>[2x]MKPHNSEKYFVKNGQPHFLISGEVHYFRINPKLWRNHLQLLKQTGADTVSTYIPWDWHEIEEDDFDFEGKTHPARNLIRFIKLCKEENLDLIVKPGPYILAEYENQGLPSWLLKKLSKNAFALDENGNVISPDLVSYLSDEFLEYTFKWYDKVMPIISKHQKEHYGPITMMQLCNEIGVFQWLSGKSDYNPKVINLYKEFIIQRYKTIEKLNSVYSTNYNSFDDLKAPSGKIKLRSDYCAYFDFHLFFREYYNKYISILKNKIRSFGINIKLTHNIPGWIYGNASELPMLISTYSEIMKNHPDIIFGLDHIPEFVSFRNAHSDLACNKILEAMQPEAPVWAAGFQAGTREHHVKAYAKDLETFYIASLAHGIKGF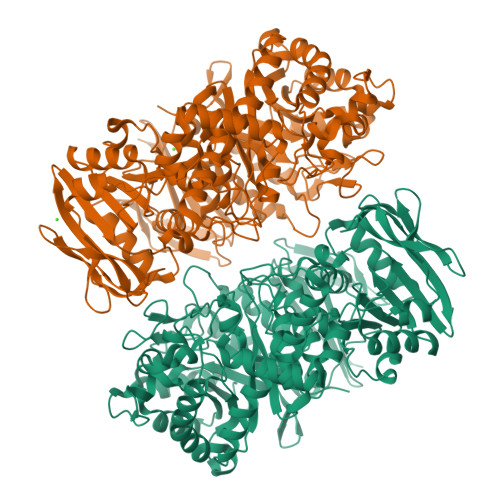NYYMFSQGINPEGKGFYGKTFYFQTALDAASNKLALYDSIKKVNRFIRKEQKDLLRTNVNSEICVGFYKPYFFTELISSQLLKEKKLNVEELGLYIDPRFLREEILFNGLLRGLQTLNYNYDVVDLENCDLKSLTAYKQLWITSAEFMDAETQNLLSEFVLNGGNLILYPAVPTLDNYLNRCEILKNNFGIEFITKDSSHKVSAFGIEDVFTAFSKKQIYNDTNSKPIAFTQENEICGIRKKIGKGELTILGFAFGYTSDEHLELIDKLVKLNKIKRELFVSDKDIQFVVRENNKSRYIFFLNYHNERKTFNYRKSSELKKKKSEEISIAPFSYKVIKENKLEHHHHHH CHOLESTERYL OLEATE | C45 H78 O2 | 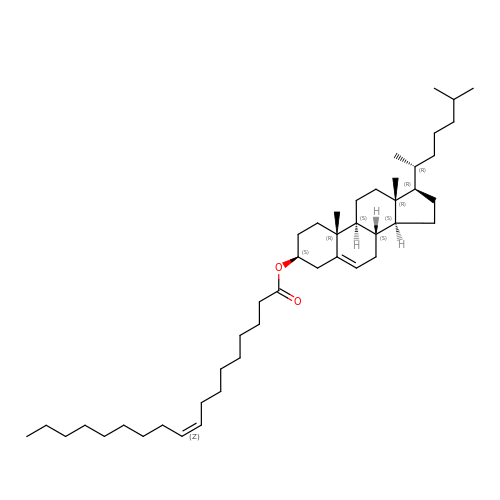RJECHNNFRHZQKU-RMUVNZEASA-N>GSMQQEALGMVETKGLTAAIEAADAMVDSANVMLVGYEKIGSGLVTVIVRGDVGAVKAATDAGAAAARNVGEVKAVHVIPRPHTDVEKILPKGIRLVKDPAANKARKEAELAAAT[6x]

The 1,2-propanediol-utilizing microcompartment is assembled from seven different types of shell proteins, one of which is PduA. It is one of the more abundant components of the shell and intriguingly can form nanotubule-like structures when expressed on its own in the cytoplasm of Escherichia coli. The majority of shell proteins consist of a single BMC domain (Pfam 00936) in each subunit and assemble into hexamers. PduA has been shown to interact with the majority of the other shell proteins and, thus, could potentially act as a scaffold for the assembly of the microcompartment.

Overexpression of K26D or V51D mutant PduAs resulted in no higher order structures being observed by TEM in the bacterial cytoplasm despite the proteins being produced in quantities suitable for crystallization and structure determination (see results below). The lysine 26 mutant is the most important to study structurally because Lys-26 is conserved in all shell proteins and contributes significantly to the interface between 2-fold related hexamers in the native crystals. Two crystal forms were obtained for this mutant using commercially available screens. There is clear electron density for residues 4–89 in nine copies of the PduA subunit across the two crystal forms, and the C-terminal residues, including the additional 23 residues, are not seen in the electron density maps. In both crystal forms, the regularity of the tiling is lost in that the K26D PduA hexamer no longer has strict 6-fold symmetry, and the separation between hexamers is greater than in native PduA sheets (67.2 Å). In the first form, strips of hexamers are formed, and in the second, sheets with rather poor hexamer-hexamer interactions are seen. It is perhaps not surprising then that no structures are seen for the K26D mutant in the bacterial cytoplasm when PduA K26D is overexpressed. For one of these mutants (K26D), crystals were obtained, and these crystals reveal more fragile hexamer-hexamer tiling than in native PduA in one crystal form (type II) and only one-dimensional tiling in the other (type I). The mutation K26D has a profound influence on the conformation of the neighboring Arg-79, such that this region of the protein no longer adopts a single conformation in the crystal, resulting in breaking of the 6-fold symmetry axis of the hexamer. This results in the imperfect tiling of PduA molecules seen in the crystals and apparent lack of tiling at all in the bacterial cytoplasm.>[6x]AKMQRSIATVSLSGTLPEKLEAIAAAGFDGVEIFENDLLYYAGSPRQVRQMCADLGIAITLFQPFRDFEGCRRDRLQKNLDRAERKFDLMQELGTDLVLVCSNVQADALGDEQLLVDDLRLLGEHAGKRGLRIGYEALAWGRHVNTYQQVWNLVRQADHPALGVILDSFHTLSLKGDPSAIRDIPGDKIFFVQMADAPILAMDVLEWSRHFRCFPGQGEMDMAGFLAPILATGYRGPLSLEIFNDGFRAAPTRQNAADGLRSLLYLEEQTRLRLEQENTPIEPGVLFSPPPASAYDGVEFLEFAVDEAVGARLGNWLKRLGFAEAGKHRSKEV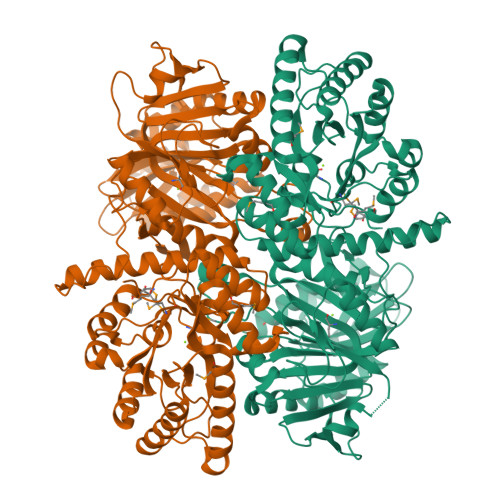QLLRQGDINIVLNAEPYSFGHNFFEAHGPSLCATALRVKDQQAALKRATAFRGQPFRGLVGPNECEVPAVRAPDGSLLYLVEQGTAGHTLYDTDFSLDNNATATGGLRRIDHMALALPAESLDSWVLFYKSLFDFAADDEVVLPDPYGLVKSRALRSQCGTLRLPLNISENRNTAIAHALSSYRGSGVHHIAFDCDDIFREVARAKLAGVPLLEIPLNYYDDLAARFDFDDEFLSELAYYNVLYDRDAQGGELFHVYTEPFEERFFFEIIQRKAGYAGYGAANVAVRLAAMAKARSGAARKPVL>RPLLIFSGQSNRPLAQAIAEALGLPLGKSTTLRFANDNLFVRYEESLREGDVFIVQSFVPPVQDHLMELLMMVDAAKGASAARVTAVIPYFSYARSDKKDAPRISITARLIADLLQTAGADRVLTMTLHSPQVHGFFKIPVDHLSAEPVIANYFATRVDLENAVVVAPDAGDLKRASALARRLGLPLAFIDKERVSDTEVRVRMLVGEVEGKTALIVDDEISTAGSLVEAVEALMQAGAKEV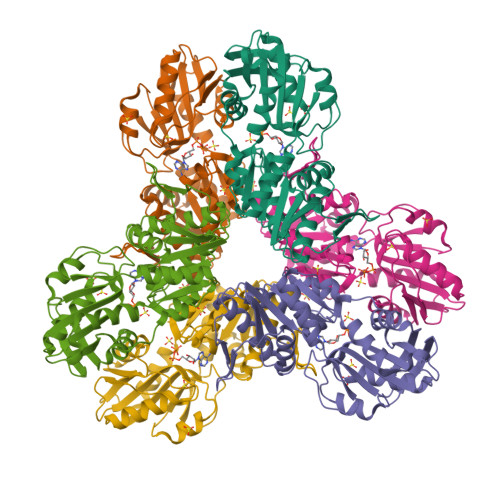YAAATHGVYVGPALDRIAKSPVKEVAATDTCPPKEGPKLRTLTVAPLFAEAIWRIHRGESVSSLFTLEHHHHHH[2x]>[3x]MKKLTIGLIGNPNSGKTTLFNQLTGSRQRVGNWAGVTVERKEGQFSTTDHQVTL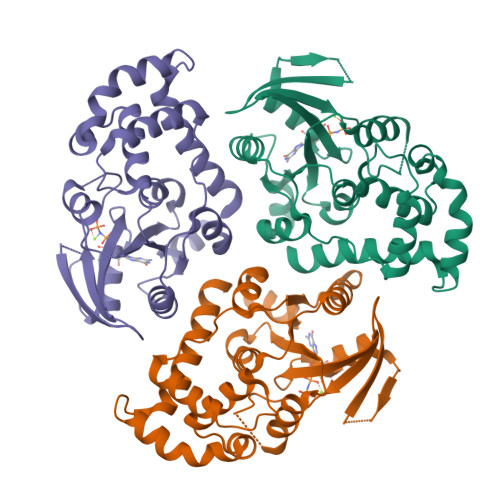VDLPGTYSLTTISSQTSLDEQIACHYILSGDADLLINVVDASNLERNLYLTLQLLELGIPCIVALNMLDIAEKQNIRIEIDALSARLGCPVIPLVSTRGRGIEALKLAIDRYKANENVELVHYAQPLLNEADSLAKVMPSDIPLKQRRWLGLQMLEGDIYSRAYAGEASQHLDAALARLRNEMDDPALHIADARYQCIAAICDVVSNTLTAEPSRF> NEQCSPQQRTTRISGRDGLCV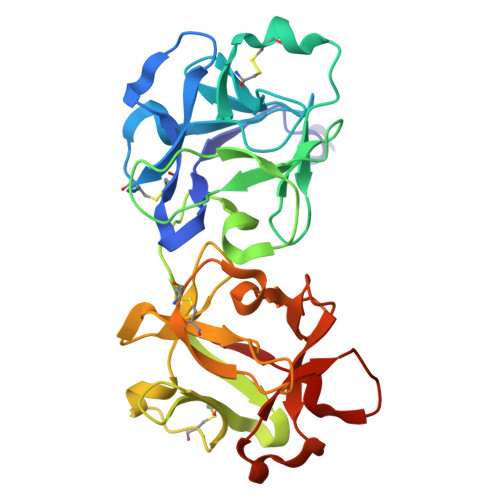DVYGALTADGSRVILYPCGQQQNQQWTFYPDNTIRSLGKCLATSALSSGSNVVITNCDYLRYDDGWMVSSSGTMMNKSSHLVLTANAATSRTNLTGENNVFAAKQAWRIGNYVEPIVTTIIGLRHMCLEATDNDTNVWLESCVKNKTKQYWALYSDDTIRVNNNRNLCVSSSTDSSSKLIVIRRCDGSINQRWVFTPQGTISNPGYEAVMDVAQNDVYLKKIVLSSATDKGNGQQWTVFY>[2x]GSHMTPISQTPGLLAEAMVDLGAIEHNVRVLREHAGHAQLMAVVKADGYGHGATRVAQTALGAGAAELGVATVDEALALRADGITAPVLAWLHPPGIDFGPALLADV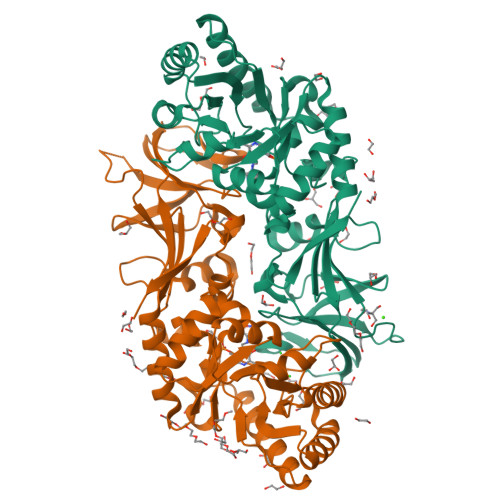QVAVSSLRQLDELLHAVRRTGRTATVTVKVDTGLNRNGVGPAQFPAMLTALRQAMAEDAVRLRGLMSHMVYADKPDDSINDVQAQRFTAFLAQAREQGVRFEVAHLSNSSATMARPDLTFDLVRPGIAVYGLSPVPALGDMGLVPAMTVKCAVALVKSIRAGEGVSYGHTWIAPRDTNLALLPIGYADGVFRSLGGRLEVLINGRRCPGVGRICMDQFMVDLGPGPLDVAEGDEAILFGPGIRGEPTAQDWADLVGTIHYEVVTSPRGRITRTYREAENR> HHHHHHPEIVDTCSLASPASVCRTKHLHLRCSVDFTRRTLTGTAALTVQSQEDNLRSLVLDTKDLTIEKVVINGQEVKYALGERQSYKGSPMEISLPIALSKNQEIVIEISFETSPKSSALQWLTPEQTSGKEHPYLFSQCQAIHCRAILPCQDTPSVKLTYTAEVSVPKELVALMSAIRDGETPDPEDPSRKIYKFIQKVPIPCYLIALVVGALESRQIGPRTLVWSEKEQVEKSAYEFSETESMLKIAEDLGGPYVWGQYDLLVLPPSF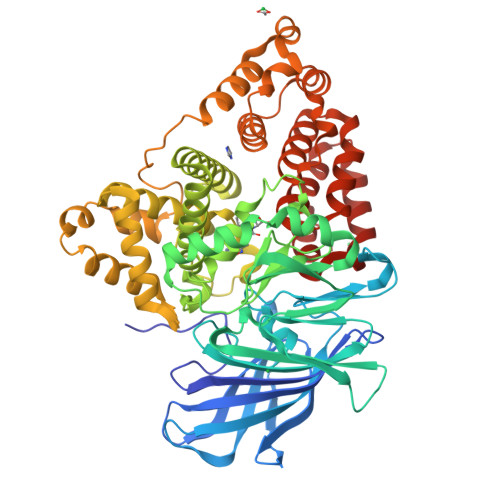PYGGMENPCLTFVTPTLLAGDKSLSNVIAHEISHSWTGNLVTNKTWDHFWLNEGHTVYLERHICGRLFGEKFRHFNALGGWGELQNSVKTFGETHPFTKLVVDLTDIDPDVAYSSVPYEKGFALLFYLEQLLGGPEIFLGFLKAYVEKFSYKSITTDDWKDFLYSYFKDKVDVLNQVDWNAWLYSPGLPPIKPNYDMTLTNACIALSQRWITAKEDDLNSFNATDLKDLSSHQLNEFLAQTLQRAPLPLGHIKRMQEVYNFNAINNSEIRFRWLRLCIQSKWEDAIPLALKMATEQGRMKFTRPLFKDLAAFDKSHDQAVRTYQEHKASMHPVTAMLVGKDLKVD> SGIVQQQNNLLRAIEAQQHLLQLTVRGIKQLQARSGGRGGWMEWDREINNYTSLIHSLI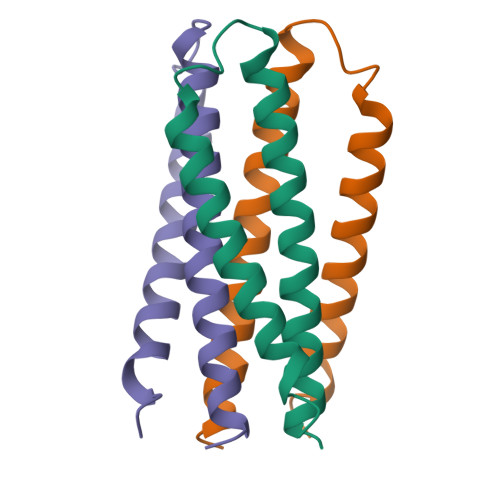EESQNQQEK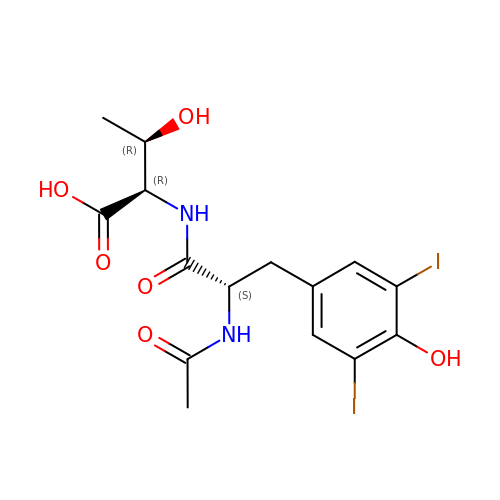N-ALPHA-ACETYL-3,5-DIIODOTYROSYL-D-THREONINE | C15 H18 I2 N2 O6 | TWMKRGDZEJLDDH-LKXWSVAYSA-N> GGSHMELPGSSMKPSGEDQAALAAGPWEECFQAAVQLALRAGQIIRKALTEEKRVSTKTSAADLVTETDHLVEDLIISELRERFPSHRFIAEEAAASGAKCVLTHSPTWIIDPIDGTCNFVHRFPTVAVSIGFAVRQELE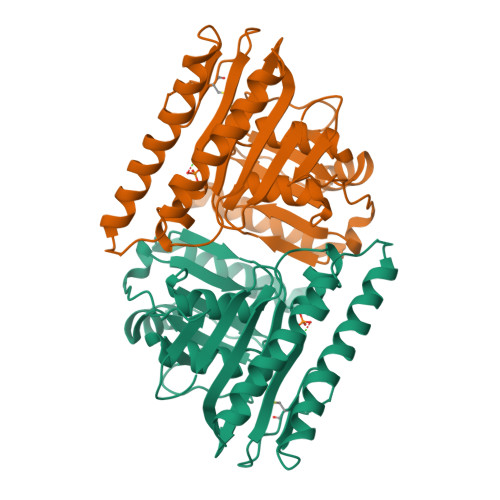FGVIYHCTEERLYTGRRGRGAFCNGQRLRVSGETDLSKALVLTEIGPKRDPATLKLFLSNMERLLHAKAHGVRVIGSSTLALCHLASGAADAYYQFGLHCWDLAAATVIIREAGGIVIDTSGGPLDLMACRVVAASTREMAMLIAQALQTINYGRDDEK> ATSTTYKVATEADDVVTRVLFDSIAHHFNLEIEYVNYPSFNDILVAIETGNADFAANITYTDLRAQRFDFSRPTNIEYTYLYSYGGLRLPELRLVGIPKGTTYGTLLKEHYPYIQQVEYEGHLEALTLLESGRVDGVVDAINQLKPMLLKGLDVQLLNDQLPIQPVSIVTPKGKHSALLGKIEKYAHSAHVQRLLRESIQKYQLDIRKQALRQSVVESGLNVQRVLRVKLENNPQYALYQPDGSVRGISADVVFQACEMLLLKCELVSNGQETWESMFDDLQDKSIDILAPITVSQQRKNLAYFSESYYHPQAILVKREHYKDDVYSNVSELVAERIGVIKDDFFEELLQQMLPNKILFSYASQEEKVQALLNKEV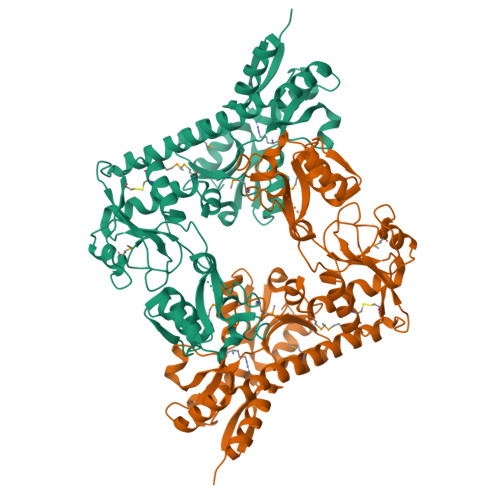DYIVLNRANFNLLLRESTEMLPIVEDTMIGSFYQYDIAIGFAKNPLGATLAPLFSRAIKMLNTEQIIHTY> GSHMGPNKMVVDLTDPNRPRFTLQELRDVLQERN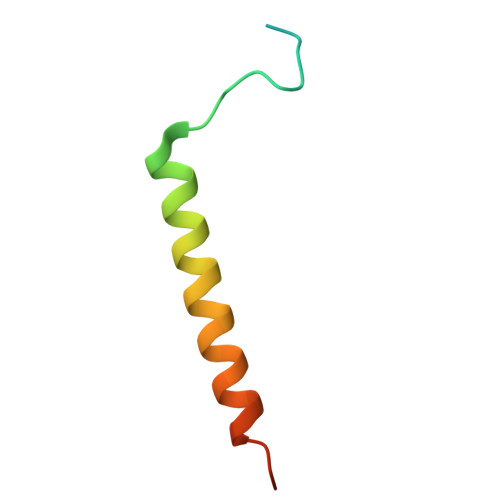KLKSQLLVVQEELQCYKSG>MGSHHHHHHRTPSDKPVAHVVANPQAEGQLQWLNRRANALLANGVELRDNQLVVPSEGLYLIYSQVLFKGQGCPSTHVLLTHTISRIAVSYQTKVNLLSAIKSPCQRETPEGAEAKPWYEPIYLGGVFQLEKGDRLSAEINRPDYLLFAESGQVYFGIIAL[6x];>ITLKYNYTVTLKDDGLYDGVFYDHYNDQLVTKISYNHETRHGNVNFRADWFNISRSPHTPGNDYNFNFWYSLMKETLEEINKNDSTKTTSLSLITGCYETGLLFGSYGYVETANGPLARYHTGDKRFTKMTHKGFPKVGMLTVKNTLWKDVKAYLGGFEYMGCSLAILDYQKMAKGKIPKDTTPTVKVTGNELEDGNMTLECTVNSFYPPDVITKWIESEHFKGEYKYVNGRYYPEWGRKSNYEPGEPGFPWNIKKDKDANTYSLTDLVRTTSKMSSQPVCVVFHDTLEAQVYTCSEGCNGELYDHLYRKTEEGEGGS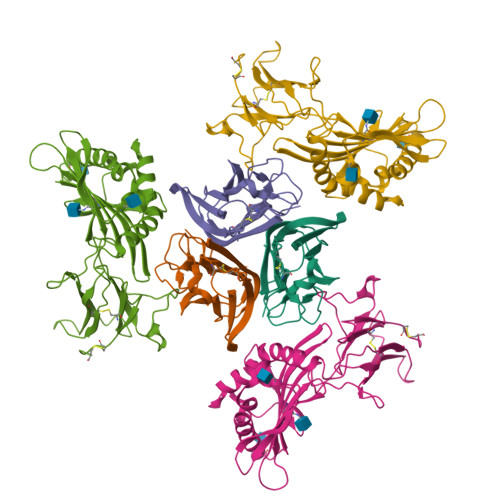HHHHHH[6x]> DMPVERILEAELAVEPKTETYVEANMGLNPSSPNDPVTNICQAADKQLFTLVEWAKRIPHFSELPLDDQVILLRAGWNELLIASFSHRSIAVKDGILLATGLHVHRNSAHSAGVGAIFDRVLTELVSKMRDMQM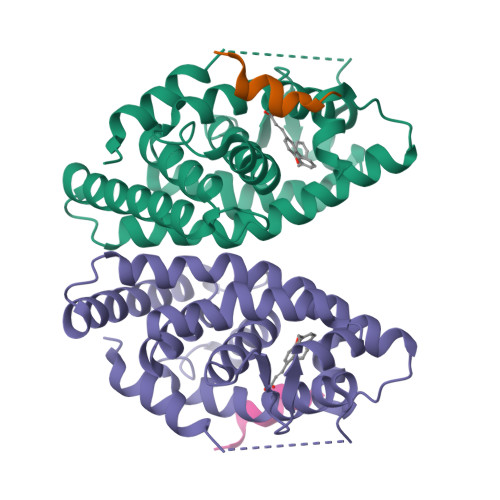DKTELGCLRAIVLFNPDSKGLSNPAEVEALREKVYASLEAYCKHKYPEQPGRFAKLLLRLPALRSIGLKCLEHLFFFKLIGDTPIDTFLMEMLEA;> KHKILHRLLQDSS> MILLDTNVISEPLRPQPNERVVAWLDSLILEDVYLSAITVAEMRLGVALLLNGKKKNVLHERMEQSILPLFAGRILPFDEPVAAIYA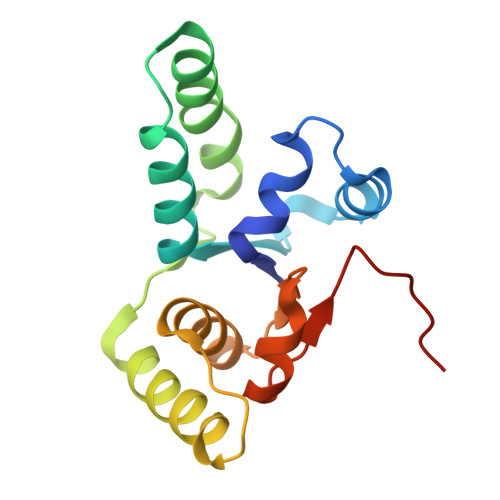QIRSYAKTHGKEIAAADGYIAATAKQHSMTVATRDTGSFFAADVAVFNPWHLEHHHHHH Na+/H+ exchangers (NHEs) are ancient membrane‐bound nanomachines that work to regulate intracellular pH, sodium levels and cell volume. Here, we report the cryogenic electron microscopy structure of NHE isoform 9 (SLC9A9) from Equus caballus at 3.2 Å resolution, an endosomal isoform highly expressed in the brain and associated with autism spectrum (ASD) and attention deficit hyperactivity (ADHD) disorders. Despite low sequence identity, the NHE9 architecture and ion‐binding site are remarkably similar to distantly related bacterial Na+/H+ antiporters with 13 transmembrane segments. The NHE9 monomer consists of 13 TMs with an extracellular N‐terminus and intracellular C‐terminus.

Surprisingly, there was no obvious density for any of the 90‐residue long C‐terminal tail regulatory domain (CTD), likely a result of its predicted dynamics and intrinsic disorder (Fig EV2A; Norholm et al, 2011; Hendus‐Altenburger et al, 2014; Pedersen & Counillon, 2019). We repeated cryo‐EM structural determination for a horse NHE9 construct lacking the entire CTD domain (NHE9 ΔCTD), which displayed similar kinetics as the close‐to‐full‐length NHE9* construct (Figs 1D and EV3 and Materials and Methods). Consistent with removal of the entire flexible CTD, 36% of the auto‐picked particles now contributed to the final 3D class with an improved EM map resolution of 3.2 Å (and EV2B and EV3). After several rounds of refinement with global and local search using ctf refine and polishing, a final resolution of 3.19 Å was achieved at gold‐standard FSC (0.143), with a local resolution range of 3.1–4.1 Å. As model building revealed only minor differences between NHE9* and NHE9 ΔCTD structures, the later was used for all subsequent analysis due to its moderately better resolution (Fig EV2C). Superimposition of NHE9* (wheat) and NHE9 ΔCTD (core transport domains (blue), dimerization domains (orange), linker helices (grey)) structures, which show only small differences in the most mobile regions. Cryo‐EM density map of the NHE9 ΔCTD homodimer with the 6‐TM core transport domains (coloured in blue), the dimer domain (coloured in orange) and the linker helix (coloured in grey). In NhaA, with 12 TMs, the dimerization interface is instead formed by interactions between an antiparallel β‐hairpin extension in a loop domain that buries a total surface area of only ~ 700 Å2 (Lee et al, 2014). In NHE9, the substrate‐binding cavity is located between the dimer and core ion‐transport domains and is open towards the intracellular side (Figs 2B and EV4A). In NHE9, the end of TM3 was observed to have moved away from the dimerization interface, exposing a hydrophobic pocket for lipids between the protomers, reminiscent of lipid binding in PaNhaP at active pH and the more distantly related citrate transporter CitS (Wohlert et al, 2014; Xu et al, 2020; Fig EV4A).

>GAVELLVFNFLLILTILTIWLFKNHRFRFLHETGGAMVYGLIMGLILRYATAPTDIESGTVYDCGKLAFSPSTLLINITDQVYEYKYKREISQHNINPHLGNAILEKMTFDPEIFFNVLLPPIIFHAGYSLKKRHFFQNLGSILTYAFLGTAISCIVIGLIMYGFVKAMVYAGQLKNGDFHFTDCLFFGSLMSATDPVTVLAIFHELHVDPDLYTLLFGESVLNDAVAIVLTYSISIYSPKENPNAFDAAAFFQSVGNFLGIFAGSFAMGSAYAVVTALLTKFTKLCEFPMLETGLFFLLSWSAFLSAEAAGLTGIVAVLFCGVTQAHYTYNNLSLDSKMRTKQLFEFMNFLAENVIFCYMGLALFTFQNHIFNALFILGAFLAIFVARACNIYPLSFLLNLGRKHKIPWNFQHMMMFSGLRGAIAFALAIRDTESQPKQMMFSTTLLLVFFTVWVFGGGTTGENLYFQ[2x]> SSQPNATLYKMSSINADFAFNLYRRFTVETPDKNIFFSPVSISAALVMLSFGACCSTQTEIVETLGFNLTDTPMVEIQHGFQHLICSLNFPKKELELQIGNALFIGKHLKPLAKFLNDVKTLYETEVFSTDFSNISAAKQEINSHVEMQTKGKVVGL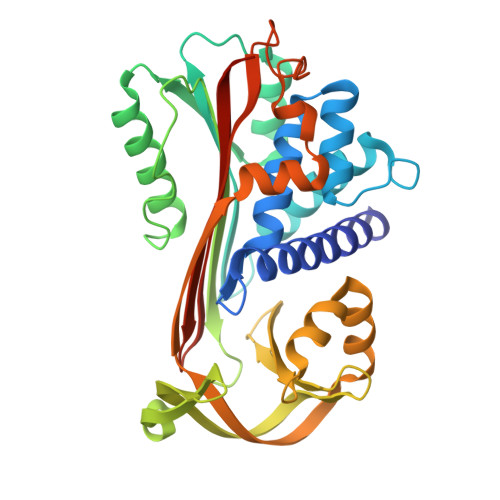IQDLKPNTIMVLVNYIHFKAQWANPFDPSKTEDSSSFLIDKTTTVQVPMMHQMEQYYHLVDMELNCTVLQMDYSKNALALFVLPKEGQMESVEAAMSSKTLKKWNRLLQKGWVDLFVPKFSISATYDLGATLLKMGIQHAYSENADFSGLTEDNGLKLSNAAHKAVLHIGEKGTEAAGAMFLEAIPRSIPNTF>X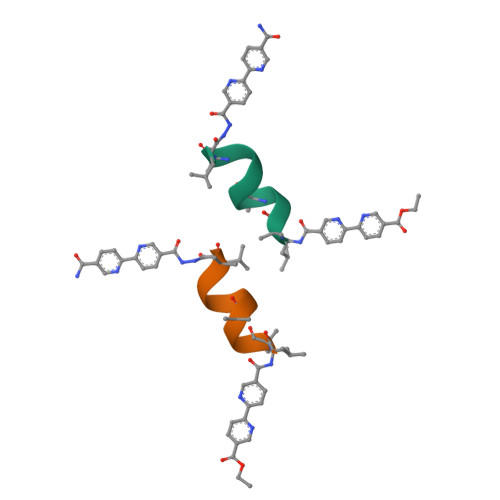LAAALHQALX[2x]N-[[2-(4-phenoxyphenyl)-1,3-thiazol-5-yl]methyl]-2-(trifluoromethyl)pyridin-4-amine 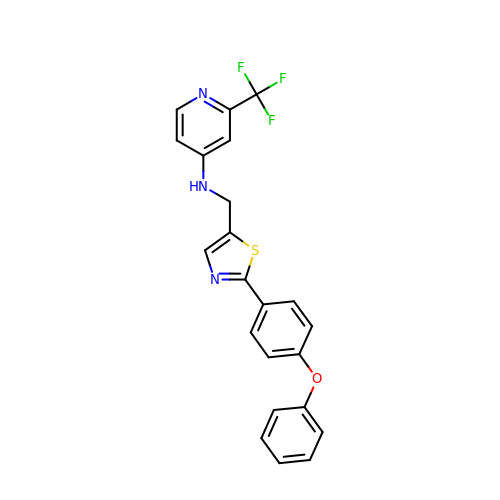| C22 H16 F3 N3 O S | GXBJUAYHTJSJOV-UHFFFAOYSA-N>MVADNIDAGVAIAVADQSSSPVGDKVELPAGNYILVGVDIDTTGRRLMDEIVQLAAYTPTDHFEQYIMPYMNLNPAARQRHQVRVISIGFYRMLKSMQTYKIIKSKSEIAALKDFLNWLEQLKTKAGPSSDGIVLIYHEERKFIPYMILESLKKYGLLERFTASVKSFANSINLAKASIGDANIKNYSLRKLSKILSLDADSLFDGNASVRAKLAFDVALQLSNSDGKPEPKSSEALENMFNAIRPFAKLVVSDVLELDIQIENLERQNSFRPVFLNYFKTTLYHRVRAVKFRIVLAENGFDLNTLSAIWAEKN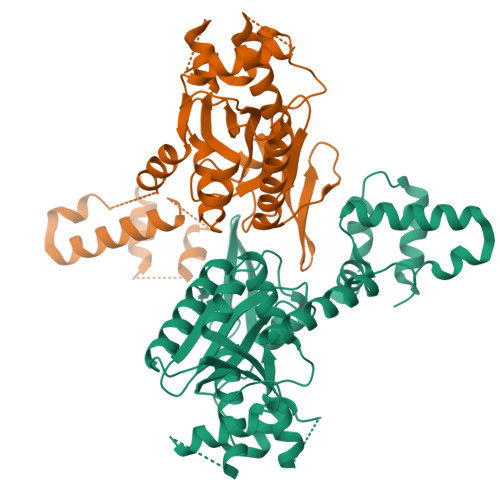IEGLDIALQSIGRLKSKDKAELLELLDSYFDPKKTTVKP[2x]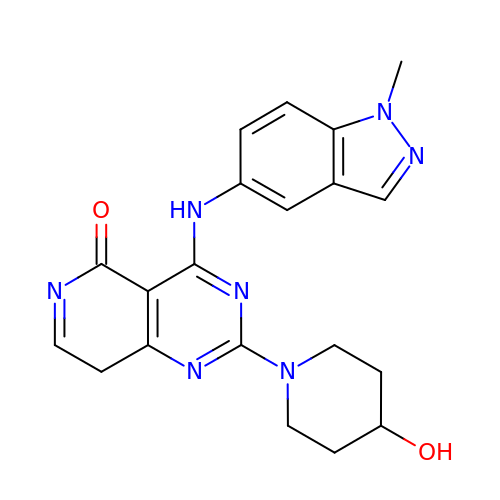4-[(1-methylindazol-5-yl)amino]-2-(4-oxidanylpiperidin-1-yl)-8H-pyrido[4,3-d]pyrimidin-5-one | C20 H21 N7 O2 | FQRDWNFNSKITIK-UHFFFAOYSA-N tert-butyl 7-[(7-methyl-1H-indazol-5-yl)carbonyl]-2,7-diazaspiro[3.5]nonane-2-carboxylate | C21 H28 N4 O3 | 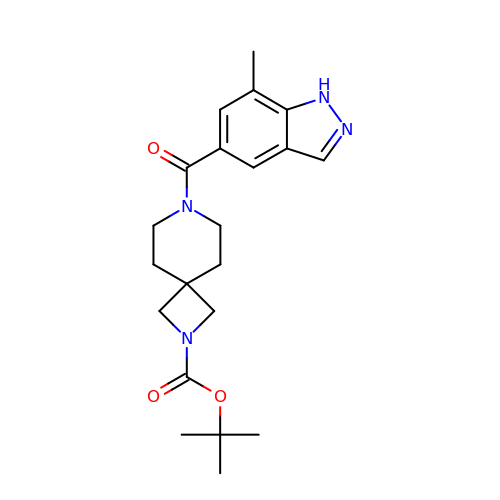YEEUURWABWXHDJ-UHFFFAOYSA-N> VGSEVS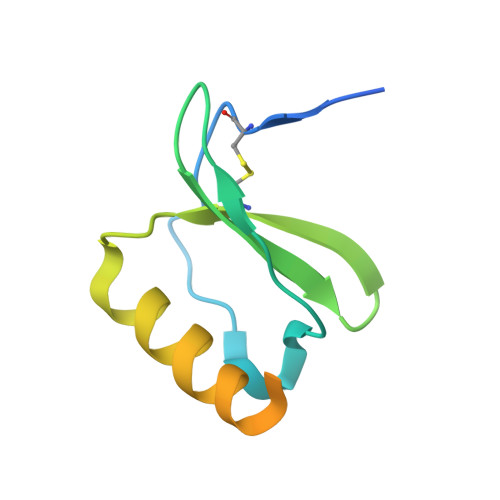DKRTCVSLTTQRLPVSRIKTYTITEGSLRAVIFITKRGLKVCADPQATWVRDVVRSMDRKSNTRNNMIQTKPTGTQQSTNTAVTLTG> GIPAELRPGTNQFLTTDDDTAAPILPGFTPTPTIHIPGEVHSLLELCRVETILEVNNTTEATGLTRLLIPVSSQNKADELCAA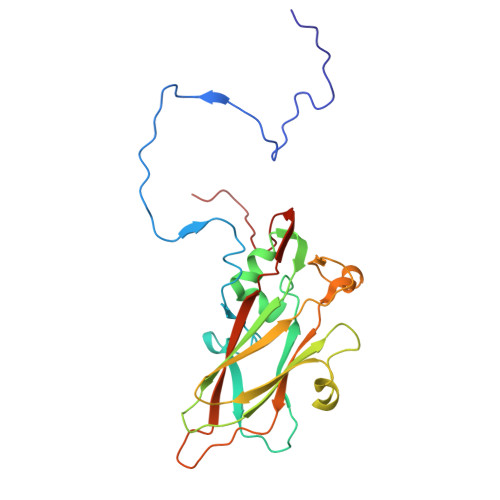FMVDPGRIGPWQSTLVGQICRYYTQWSGSLKVTFMFTGSFMATGKMLVAYSPPGSAQPANRETAMLGTHVIWDFGLQSSVSLVIPWISNTHFRTAKTGGNYDYYTAGVVTLWYQTNYVVPPETPGEAYIIAMGADLYKFTLKICKDTDEVTQQAVLQ> GSHMENYHAGPGISKSQLDDIADTPALYLWRKNAPVDTTKTKTLDLGTAFHCRVLELEEFSNRFIVAPEFNRRTNAGKEEEKAFLMECASTGKTVITAEEGRKIELMYQSVMALPLGQWLVESAGHA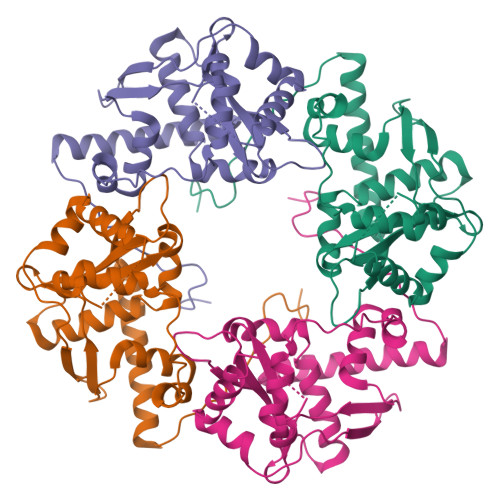ESSIYWEDPETGILCRCRPDKIIPEFHWIMDVKTTADIQRFKTAYYDYRYHVQDAFYSDGYEAQFGVQPTFVFLVASTTIECGRYPVEIFMMGEEAKLAGQQEYHRNLRTLSDCLNTDEWPAIKTLSLPRWAKEYAND> HECQCQCGSCKNNEQCQKSCSCPTGC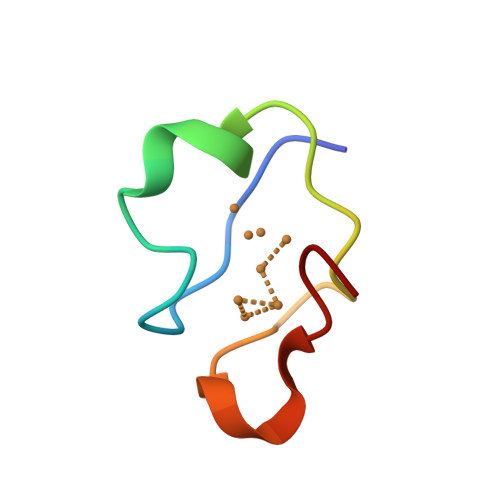NSDDKCPCGN> PNGQTKPLPALKLALEYIVPCMNKHGICVVDDFLGKETGQQIGDEVRALHDTGKFTDGQLVSQKSDSSKDIRGDKITWIEGKEPGCETIGLLMSSMDDLIRHCNGKLGSYKINGRTKAMVACYPGNGTGYVRHVDNPNGDGRCVTCIYYLNKDWDAKVSGGILRIFPEGKAQFADIEPKFDRLL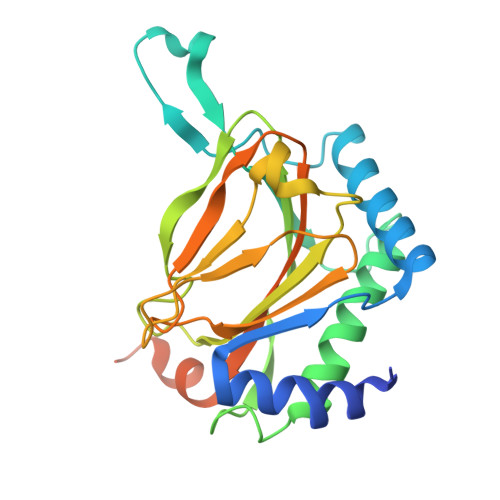FFWSDRRNPHEVQPAYATRYAITVWYFDADERARAKVKYLTGEKGVRVELNKPSDSVGKDVF>GSIGSNSIDLITKYEPIFLGSGIYFLRPFNTDERDKLMVTDNAMSNWDEITETYYQKFGNAINKMLSLRLVSLPNGHILQPGDSCVWLAEVVDMKDRFQTTLSLNILNSQRAEIFFNKTFTFNEDNG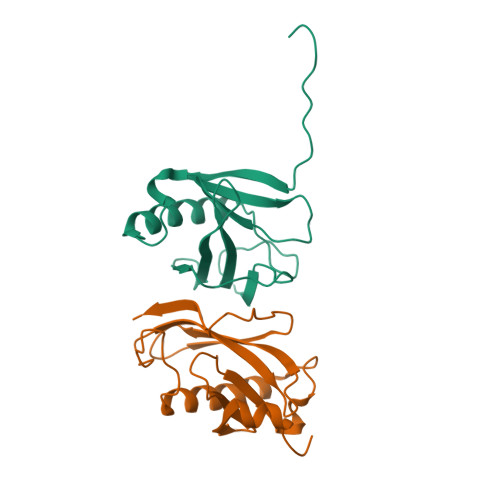NFLSYKIGDHGESTELGQITHSNKADINTAEIRS[2x]>[2x]AQEVFRNTVTGEALDVEGQAPKEGRDTPAV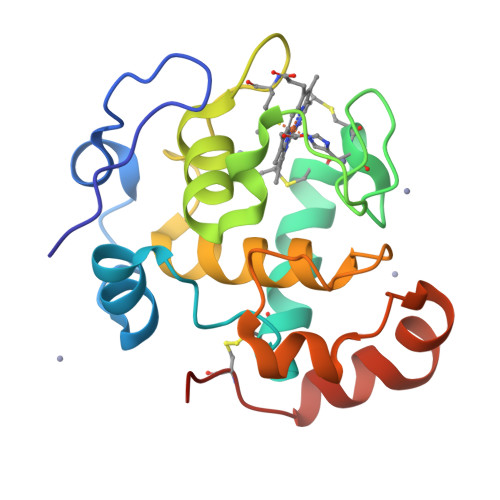KQFMQTGVDPYVEVAGCLPKGEEIYLESCSGCHGHIGEGKVGPGLNDSYWTYPKNTTDKGLFETIFGGANGMMGPHGQDLELDNMLKLIAWIRHIQKDDVADADWLSDEQKKNFKPFDIKAWEATGKAAAEKAQCKISGN>LATLLGLIGGFAFVIMAMVLGGSIGMFVDVTSILIVVGGSIFVVLMKFTMGQFFGATKIAGKAFMFKADEPEDLIAKIVEMADAARKGGFLALEEMEINNTFMQKGIDLLVDGHDADVVRAALKKDIALTDERHTQGTGVFRAFGDVAPAMGMIGTLVGLVAMLSNMDDPKAIGPAMAVALLTTLYGAILSNMVFFPIADKLSLRRDQETLNRRLIMDGVLAIQDGQNPRVIDSYLKNYLNEGKRALEID[3x];>MDLATLLGLIGGFAFVIMAMVLGGSIGMFVDVTSILIVVGGSIFVVLMKFTMGQFFGATKIAGKAFMFKADEPEDLIAKIVEMADAARKGGFLALEEMEINNTFMQKGIDLLVDGHDADVVRAALKKDIALTDERHTQGTGVFRAFGDVAPAMGMIGTLVGLVAMLSNMDDPKAIGPAMAVALLTTLYGAILSNMVFFPIADKLSLRRDQETLNRRLIMDGVLAIQDGQNPRVIDSYLKNYLNEGKRALEI[2x];>[2x]PPPGLPLWMGTFADLMSLLMCFFVLLLSFSEMDVLKFKQIAGSMKFAFGVQ

Vibrio spp. are highly motile bacteria responsible for various human diseases, the polar flagella of which are exclusively driven by sodium-dependent stator units (PomAB). The flagellar stator unit uses the transmembrane ion motive force (IMF) to generate mechanical torque to rotate the flagellum, which is employed by many bacteria to direct their locomotion in liquid environment or on viscous surfaces to a favorable niche. PomAB assembles the characteristic bell shape of the stator unit family, with conserved 5:2 subunit stoichiometry and overall architecture. Five PomA molecules arrange pseudo-symmetrically around two PomB, with each PomA subunit comprising four transmembrane helices (TM1-TM4) folded into two radial layers.

Single-particle analysis yielded an overall resolution of VaPomAB in Lauryl Maltose Neopentyl Glycol (LMNG) detergent of ~2.5 Å, with the cryo-EM map of sufficient quality to build an atomic model for most of the protein complex. The local resolution corresponding to the inner transmembrane domain approaches 2 Å, with clear density for non-protein molecules, allowing us to model water molecules and ions, as well as residue side chains isomers. The plugged motifs from two PomB chains are fully resolved in our PomAB structure, where they are positioned on the top of the periplasmic side of the stator unit, consistent with a plugged autoinhibited state. The PomAB structure shows that the D24 of two PomB chains sit in different environments; D24 of Pom B chain 1 interacts with PomA, which we refer to as an engaged state; while D24 of PomB chain 2 points towards the cytoplasmic domain and breaks the interaction with PomA, which we refer to as a disengaged state. Examination of the high-resolution density map in the vicinities of these two aspartates reveals nonresidue densities. In site 2, near the disengaged PomB D24, which is more flexible as indicated by the slightly blurred EM density of its acidic side chain, a globular density is well coordinated by oxygen atoms exclusively contributed by PomA TM3 and TM4: side chain hydroxyl groups of T158, T185 and T186, and exposed backbone carbonyl groups of G154 and A182, with an average distance between the density center and associated oxygen of 2.33 Å. To further validate the model, we performed two explicit solvent all-atom MD simulations (1 µs for each) and observed that the Na+ ion in site 1 was very stable, but the other Na+ ion in site 2 rapidly moved to an intermediate site formed by the side chain of D24, T158, and T186 and subsequentially to a location symmetric to site 1, and finally released to the cytoplasmic space.>[2x]ATQGQVITCKAAVAYEPNKPLVIEDVQVAPPQAGEVRIKILYTALCHTDAYTWSGKDPEGLFPCILGHEAAGIVESVGEGVTEVQAGDHVIPCYQAECRECKFCKSGKTNLCGKVRSATGVGIMMNDRKSRFSVNGKPIYHFMGTSTFSQYTVVHDVSVAKIDPTAPLDKVCLLGCGVPTGLGAVWNTAKVEPGSNVAIFGLGTVGLAVAEGAKTA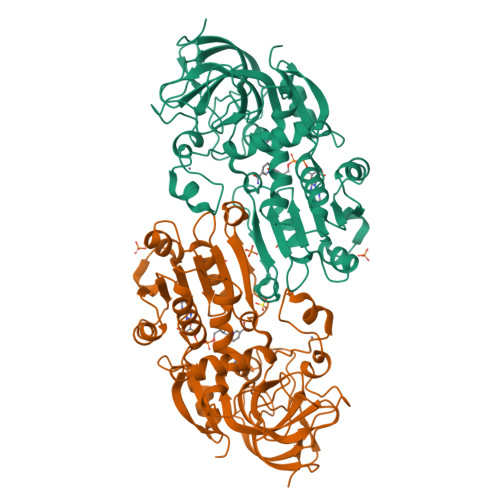GASRIIGIDIDSKKYETAKKFGVNEFVNPKDHDKPIQEVIVDLTDGGVDYSFECIGNVSVMRAALECCHKGWGTSVIVGVAASGQEISTRPFQLVTGRVWKGTAFGGFKSRTQVPWLVEKYMNKEIKVDEYITHNLTLGEINKAFDLLHEGTALRAVLDTSK AMA1, a type I transmembrane protein, is conserved across all Apicomplexans and its knockdown has been shown to markedly reduce invasion. Recently, Toxoplasma sporozoites were subjected to detailed transcriptomic and proteomic analyses. It was found that, in addition to the well-characterized “generic” AMA1 and RON2, sporozoites also express two paralogues dubbed sporoAMA1 and sporoRON2, respectively, that are not expressed at detectable levels in tachyzoites or bradyzoites. To better understand the mutually exclusive nature of the interaction between the sporozoite and generic AMA1/RON2 pairings, we set out to solve the crystal structure of apo sporoAMA1 and of sporoAMA1 bound to a portion of sporoRON2-D3 (sD3). The results presented here demonstrate that invasion of Toxoplasma sporozoites depends on the interaction of two previously uncharacterized proteins, sporoRON2 and sporoAMA1.

Overall, the structure of apo sporoAMA1 conforms to the expected three-domain architecture observed for other AMA1 structures, but reveals several divergent substructures including a network of apical surface loops that provide an unexpected degree of integration with the apical groove. In particular, apical loops 1 and 2 of domain I and the extended loop of domain II (DII loop) cover the region occupied by RON2 in previously determined AMA1/RON2 co-structures from both T. gondii and P. falciparum. In addition, sporoAMA1 loop 2 is slightly longer than the analogous loop in generic AMA1 and has an N-linked glycosylation at Asn230 that is positioned atop the groove (Fig. 3B; note that while generic AMA1 has been reported to be naturally N-glycosylated in tachyzoites, no information exists on sporoAMA1 in this regard but it does have a consensus N-linked site which is efficiently N-glycosylated in the insect cells used to generate the recombinant sporoAMA1 studied here). Loop 2 folds in over the top of the groove, and positions Pro227 directly over the tip of the DII loop, which appears to compensate for the lack of the central anchoring tyrosine observed in generic AMA1 (sporoAMA1 Ser252; generic AMA1 Tyr230), with Pro227 effectively pinning DII loop Phe376 and Trp377 into the base of the apical groove. Based on the degree to which the apical groove of sporoAMA1 is guarded, numerous specific interactions between sporoAMA1 and sporoRON2, particularly in the predicted initial binding site at the cysteine loop, are likely to be required to overcome the energy barriers of DI apical loop rearrangement and displacement of the DII loop.

>GSAMGQNPWATTTAFADFMKRFNIPQVHGSGIFVDLGRDTEGYREVGGKCPVFGKAIQMHQPAEYSNNFLDDAPTSNDASKKPLPGGFNNPQVYTSGQKFSPIDDSLLQERLGTAGPKTAIGRCALYAYSTIAVNPSTNYTSTYKYPFVYDAVSRKCYVLSVSAQLLKGEKYCSVNGTPSGLTWACFEPVKEKSSARALVYGSAFVAEGNPDAWQSACPNDAVKDALFGKWEDGQCVPFDTKTSVQSDQATNKEECWKRVFANPLVASDAPTTYPEAAQKNWNDFWPVHEQSSPKSGGFGANWANFYLEKESGETICAIFDQVPDCFAPITGAVAYTALGSSTEVNLPQCDSASFIPIEGPCNNCVQVVTECVGNQFDQTSKACCTEPEAAALVPR[12x]> MALDRPDRSGAVRVSAPARLSFTAISLDGSSLRRNGIAAMAVDRPGLTAEVREAADGIVAVTGTAEETARELAAALEALRKLWDGPAARVDVLEALPQHSGFGSKTSTLLAVGHAYGRLCGVEPDLRELARTLGRGRTSGASTGLSAYGGFLVDGGHVNPPDFAEAPQKYLRPSRFAQQVA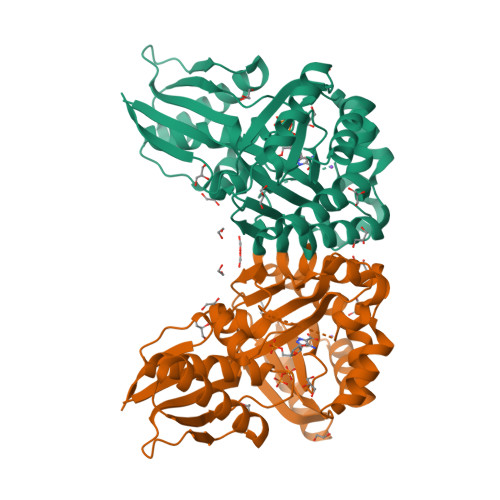PPKPVVRLDFPDWPVLVLLTHGRHLGGQEELEWFHSVAPIPAEESWRTSHLVFMGLAPAVLEQDFDAFCAAVNEITFTGHFKQAQIAFQGDAVADVLEAGRAAPSVDAIALSVTGPACFAFTKRPEDAERWAWELKNRGLIRDFWFTRANNQGLATTVVS>[2x]SLENAGSRPFLADFNGFSYLELKGLHTFERDLGEKMALEMVFLARGPSGLLLYNGQKTDGKGDFVSLALHNRHLEFRYDLG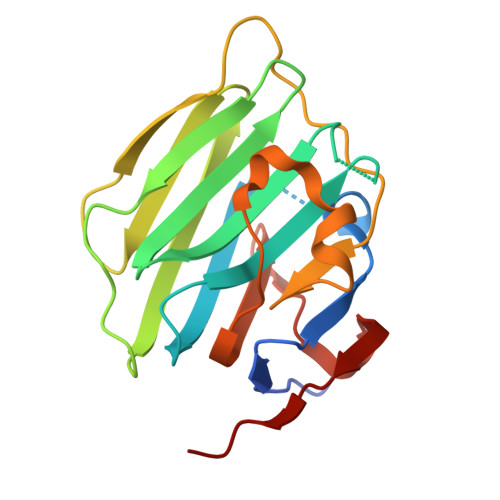KGAAIIRSKEPIALGTWVRVFLERNGRKGALQVGDGPRVLGESPVPHTMLNLKEPLYVGGAPDFSKLARGAAVASGFDGAIQLVSLRGHQLLTQEHVLRAVDVAPFAG> GP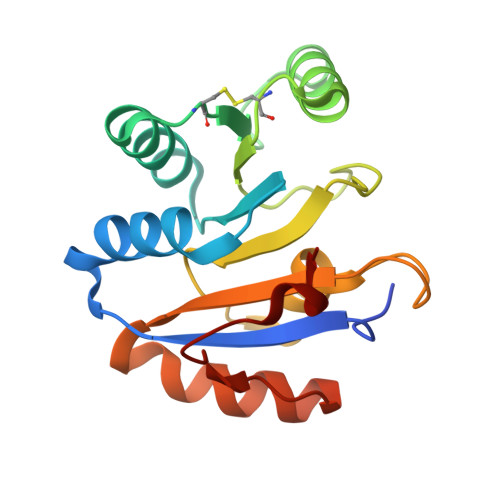HMELTLKGVTQYYAFVQERQKVHCLNTLFSKLQINQSIIFCNSTQRVELLAKKITELGYCCYYIHAKMAQAHRNRVFHDFRQGLCRNLVCSDLFTRGIDVQAVNVVINFDFPRMAETYLHRIGRSGRFGHLGIAINLITYEDRFDLHRIEKELGTEIKPIPKVIDPALYV>GSMTGAS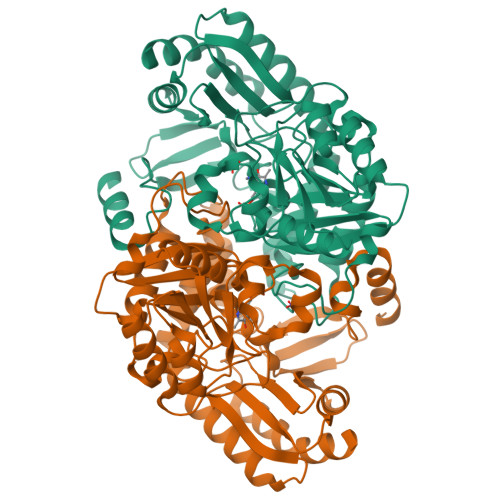TTTATMRQRWQAVMMNNYGTPPIALASGDGAVVTDVDGRTYIDLLGGIAVNVLGHRHPAVIEAVTRQMSTLGHTSNLYATEPGIALAEELVALLGADQRTRVFFCNSGAEANEAAFKLSRLTGRTKLVAAHDAFHGRTMGSLALTGQPAKQTPFAPLPGDVTHVGYGDVDALAAAVDDHTAAVFLEPIMGESGVVVPPAGYLAAARDITARRGALLVLDEVQTGMGRTGAFFAHQHDGITPDVVTLAKGLGGGLPIGACLAVGPAAELLTPGLHGSTFGGNPVCAAAALAVLRVLASDGLVRRAEVLGKSLRHGIEALGHPLIDHVRGRGLLLGIALTAPHAKDAEATARDAGYLVNAAAPDVIRLAPPLIIAEAQLDGFVAALPAILDRAVGAP[4x]> MGHHHHHHGSGSNRLDGKVAIITGGTLGIGLAIATKFVEEGAAVMITGRHSDVGEKAAKSVGTPDQIQFFQHDSSDEDGWTKLFDATEKAFGPVSTLVNNAGIAVNKSVEETTTAEWRKLLAVNLDGVFFGTRLGIQRMKNKGLGASIINMSSIEGFVGDPSLGAYN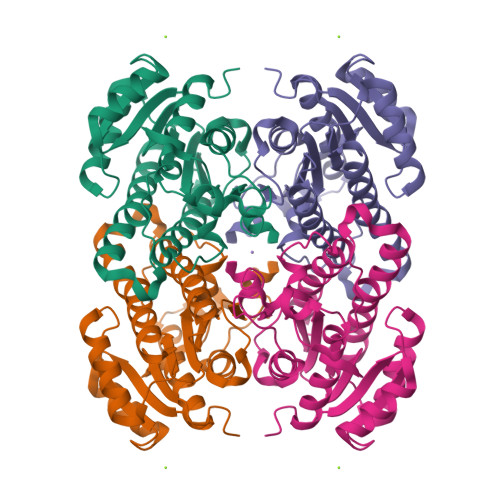ASKGAVRIMSKSAALDCALKDYDVRVNTVHPGYIKTPLVDDLPGAEEAMSQRTKTPMGHIGEPNDIAYICVYLASNESKFATGSEFVVDGGYTAQ> GAMEPQVTLNVTFKNEIQS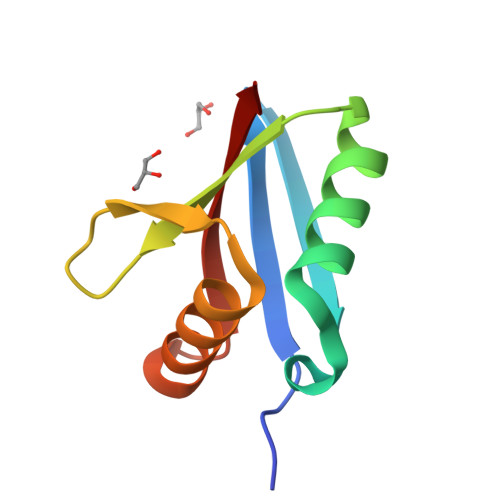FLVSDPENTTWADIEAMVKVSFDLNTIQIKYLDEENEEVSINSQGEYEEALKMAVKQGNQLQMQVHEG>MADGGESSNANAGEGTSGGGGSGPLALTGGSRAGGTIGGGGAGSVGFSTGGWTAGTYFSDNKVVTNQTRQFLTPIYNGHTYKALQADDLTNENDKSKWNGITTPWGYFNFNCYASHFSPQDWQRMCNEYKRWRPKRLRVQIYNLQLKTIQSNGADTQYNNDLTAAVHILVDGSHQFPWAQHPWDDTCAPELPYVIYKTPQYAYFQNLAGLANNVGTNSANKFLKMNTPLYVLETMSHEVLRTGEDTSFEFEMSSGWVDNQTNFCPPQLDFNPLHDTRRVAPRATNNTTQYAPYPKFKKPSNWVPGPGMAYPGRGEADGKRPAPMTVTLRPNTFIDAGNNTTDRFQQASYQEWKPTDDTIIGQSINVGPINCAATDPDAVTTAADAEDDVANPNTDKVSSHRYSIDMTRWNAIQINVRRNNGTPETTQIYRHYLYPMQAWNSNQIDRYTPIWDKVPNTEWHTMLASSDGTLPMTHPPGTIFIKCSKIPVPSENNADSYLNIYCTGQVSYEIEWECERYNTKNWRPELRVDPKNWTDPNNYNLNTQGGYIVNEELYET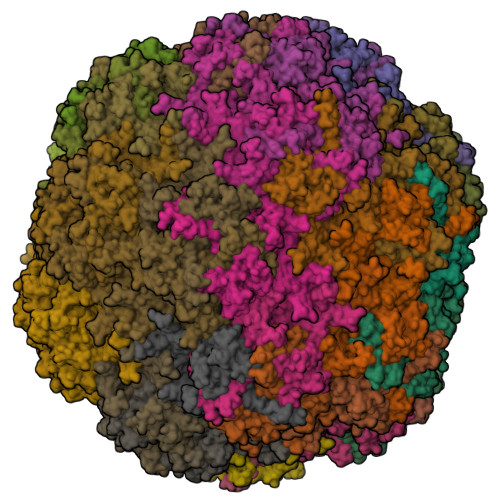MPTKIGINRVN[60x]>GSAKDPKSTVASSTTEDLKVSTTAGAAAGTYKINVTQLAAAQSLATKTTFATTKEQLGDTSVTSRTIKIEQPGRKEPLEIKLDKGDTSMEAIRDAINDADSGIAASIVKVKENEFQLVLTANSGTDNTMKITVEGDTKLNDLLAYDSTTNTGNMQELVKAENAKLNVNG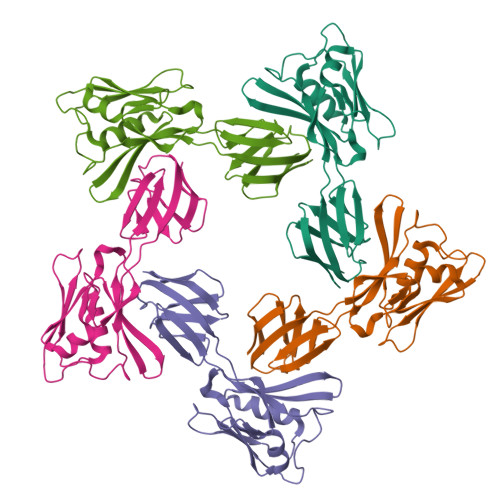IDIERQSNTVTDAPQGITLTLTKKVTDATVTVTKD[5x]> HHHMLTYGAPFNFPRWIDEHAHLLKPPVGNRQVWQDSDFIVTV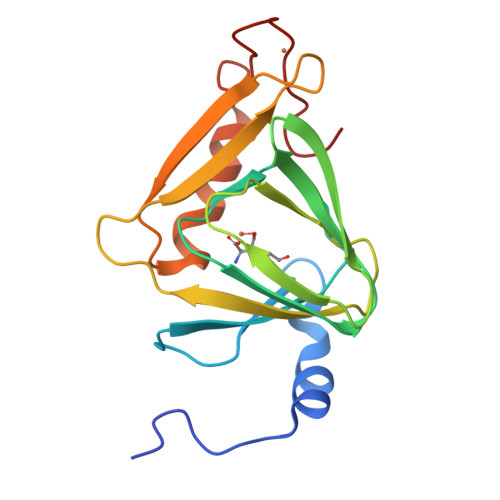VGGPNHRTDYHDDPLEEFFYQLRGNAYLNLWVDGRRERADLKEGDIFLLPPHVRHSPQRPEAGSACLVIERQRPAGMLDGFEWYCDACGHLVHRVEVQLKSAVTDLPPLFESFYASEDKRRCPHCGQVHPGRAA>WSHPQFEKTAGRRKVQVSYVIRDEVEKYNRNGVNALQLDPALNRLFTAGRDSIIRIWSVNQHKQDPYIASMEHHTDWVNDIVLCCNGKTLISASSDTTVKVWNAHKGFCMSTLRTHKDYVKALAYAKDKELVASAGLDRQIFLWDVNTLTALTASNNTVTTSSLSGNKDSIYSLAMNQLGTI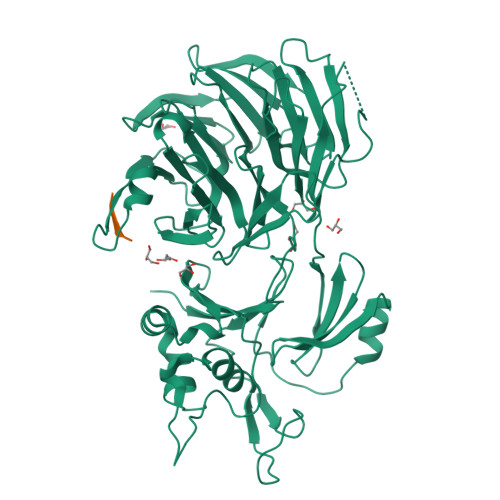IVSGSTEKVLRVWDPRTCAKLMKLKGHTDNVKALLLNRDGTQCLSGSSDGTIRLWSLGQQRCIATYRVHDEGVWALQVNDAFTHVYSGGRDRKIYCTDLRNPDIRVLICEEKAPVLKMELDRSADPPPAIWVATTKSTVNKWTLKGIHNFRASGDYDNDCTNPITPLCTQPDQVIKGGASIIQCHIFNDKRHILTKDTNNNVAYWDVLKACKVEDLGKVDFEDEIKKRFKMVYVPNWFSVDLKTGMLTITLDESDCFAAWVSAKDAGFSSPDGSDPKLNLGGLLLQALLEYWPRTHVNPMDEEENEVNHVNGEQENRVQKGNGYFQVPPHTPVIFGEAGGRTLFRLLCRDSGGETESMLLNETVPQWVIDITVDKNMPKFNKIPFYLQPHASSGAKTL[2x]>[2x]ATPLTSLGSEQAMFHGKHQPGITTPMQARGHLVAFD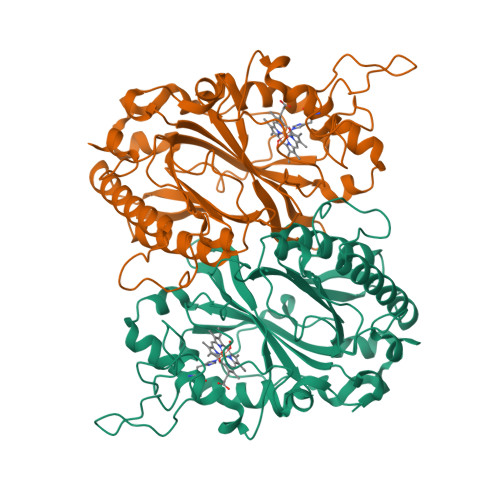LAAGAGRKEAAALLRRWSDTARRLMAGEPAGSRDTDVARDAGPSSLTVTFGFGHSFFGRTGLEKQRPVALDPLPDFSSDHLDKNRSNGDLWVQIGADDALVAFHALRAIQRDAGAAARVRWQMNGFNRSPGATAHPMTARNLMGQVDGTRNPKPGEADFDRRIFVPEEPEAGKGGPAWMANGSYVVVRRIRMLLDDWEELSLKAQEDVIGRRKSDGAPLSGGSGATESTEMDLEKTDGSGELVVPINAHARITRPDQNGGAAMVRRPFSYHDGFDADGVPDAGLLFVCWQADPLRGFVPVQRKLDRGDALSQFIRHEASGLFAVPGGAAEGEYVGQRLLEG> AMAPAKKSEELVAEAHNLCTLLENAIQDTVREQDQSFTALD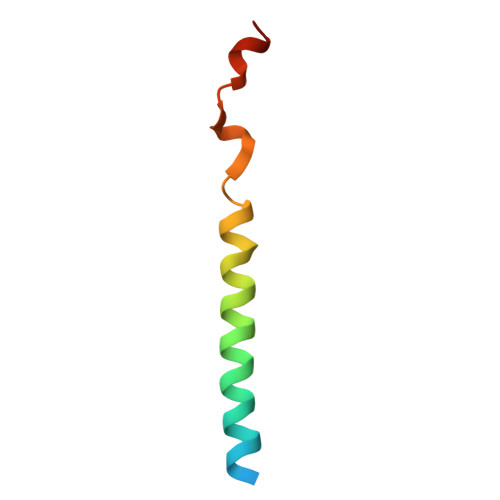WSWLQTE>SNARYRATHERVFTILESFDNTRPRIDVERAKYFTESMKATEGQPLPLRWAKALMHIAENMTVYIDDHQLICGRAGYQGRYGVLYPELDGDFLGTAIEDLPNRAESPFAITPAAAAVVVEEIAPFWKGKTYHEALNLALPADVHKLTYDDPQGLMSRFIVNETSSFRSSIQWVHDYEKVLKRGFRSIKEEALEKIAALDPMSPCDNVEKRPFLEAIVIVCDAIILWAKRHAKLAAELAAKETDPTRKRELETMAEICAWVPENPARTFHEAVQAQWFTQVFSRIEQKTGTIVSNGRMDQYFWPFYEKDLAEGRITEDSALELLECMWVGMAQYVDLYISPTGGAFNEGYAHWEAVTIGGQTPEGRDATNDLTYLFLKSKREFPLHYPDLAARIHSRSPERYLWEVAETIKDGSGFPKLINDEEVVPLYVSKGATFAEALDYAVSGCTEARMPNRDTYTSGGAYINFAAALEMVLYNGKMLKYGDTDLGAHTGDPCEFKTWEEFWNAYVTQHHLFLKTAFVQQHIINNLRARHFAQPMGSSLHDLCMKHCLDLHT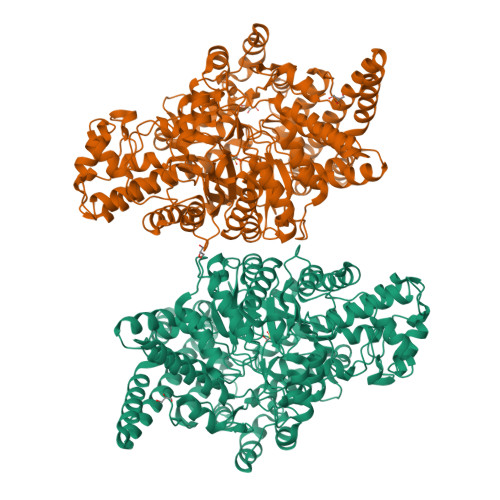PQIPEGINLGYFEYMGFGTVVDSLSAIKKLVFEDKKLTMGELIEALKCNFEGKEDIQQLLKSAPCYGNNDDYADSIARDIDALSVKYGRRYSPELGMHNDVRYVPFTSHVPFGRVVSATPNGRKAWSALSDGSSASHGADVNGPTAILQSNFNSKNYGMRDRAARMLNIKFTPKCVEGEEGSQKLVSFIRTFCDLKLWHVQFNVINKETLLAAQRDPEKYRNLIVRIAGYSAYFVDLSPDLQNDLIARTGHDVM[4x]>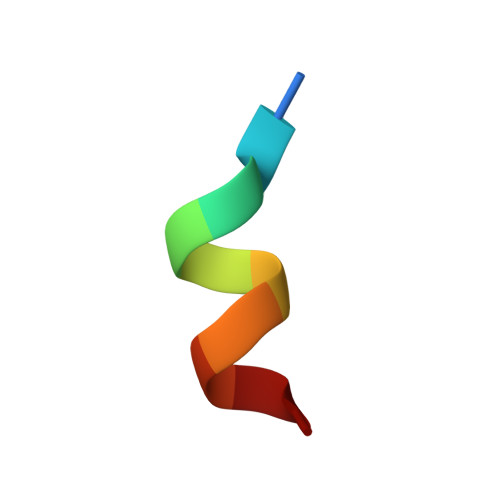 NHPMLMNLLK>[8x]MALNVGPGGGSPVSTVEDTGRVELTPQEAAKVATTRCICYSTTQYVKDFLAGPMQKVFTDTYFVEPPLDKDTAQLARGYDVAVLFVNDRADASVIKELAK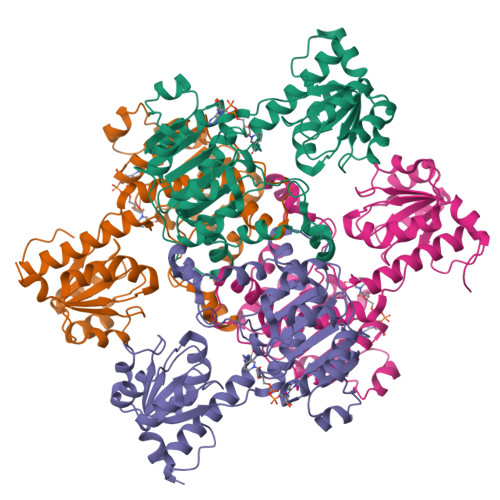AGVKLIALRCAGFDRVDLHACAEHGVRVVRVPTYSPESVAEHAVALIFALNRHLTDAYIRVRMGNYSLSGLVGVEMRHKVVGVVGTGAIGQQAARILKGIGCKVFAYDIKPNPAVEAMGIPYVSLDELLAMSDIVTLHCPLLPSTRQLINKESIQKMKKGVMLINVSRGGLIDSAALFDALESGQIGALGLDVYENEGGLFFVDHTKFDPSVRMQKWDRQFRTLLSYPQVLVTPHTAFLTEEALNNICTTTIQNIADYVLDRPLGNEVKAQPAPAGKTLEHHHHHH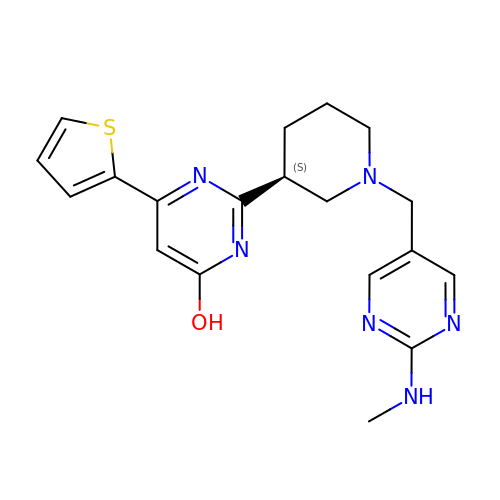(6M)-2-[(3S)-1-{[2-(methylamino)pyrimidin-5-yl]methyl}piperidin-3-yl]-6-(thiophen-2-yl)pyrimidin-4-ol | C19 H22 N6 O S | ZSXCVAIJFUEGJR-AWEZNQCLSA-N>GAQNEKNMYSYKKIGNKYIVSINNHTEIVKALNAFCKEKGILSGSINGIGAIGELTLRFFNPKTKAYDDKTFREQMEISNLTGNISSMNEQVYLH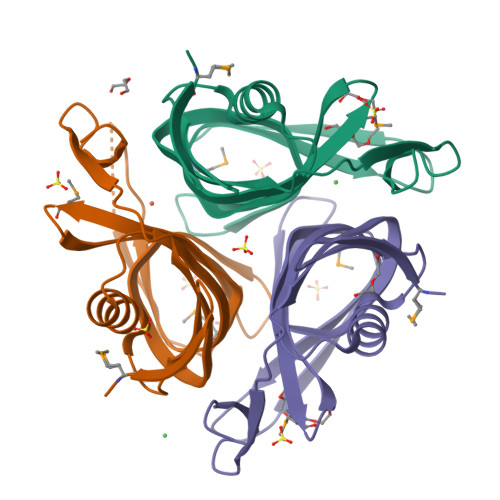LHITVGRSDYSALAGHLLSAIQNGAGEFVVEDYSERISRTYNPDLGLNIYDFER[3x]>[2x]GENSDNLTHCRLFEFRLCLLEC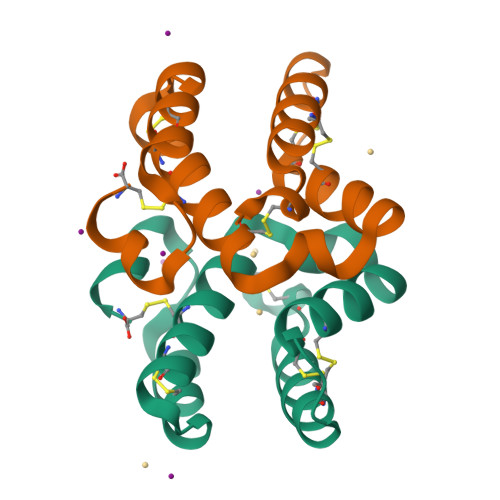MSLTLDHCYARCTTVITQIHGSDTNRFDCTIFKTCYYRCYVLGKTEDHCWKGTATSVTGDVGDLEFC> MKIEEVKSTTKTQRIASHSHVKGLGLDESGLAKQAASGLVGQENAREACGVIVELIKSKKMAGRAVLLAGPPGTGKTALALAIAQELGSKVPFCPMVGSEVYSTEIKKTEVLMENFRRAIGLRIKETKEVYEGEVTELTPCETENPMGGYGKTISHVIIGLKTAKGTKQLKLDPSIFESLQKERVEAGDVIYIEANSGAVKRQGRCDTYATEFDLEAEEYVPLPKGDVHKKKEIIQDVTLHDLDVANARPQGGQDILSMMGQLMKPKKTEITDKLRGEINKVVNKYIDQGIAELVPGVLFVDEVHMLDIECFTYLHRALESSI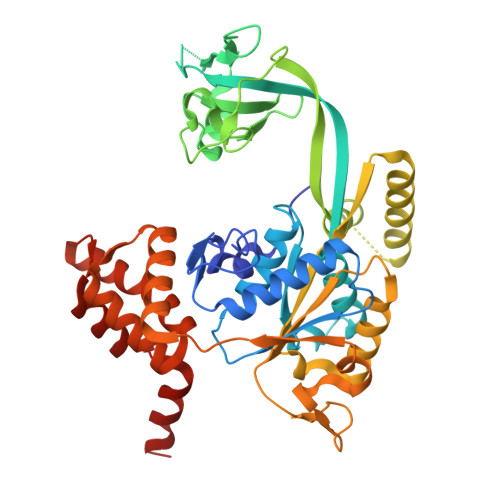APIVIFASNRGNCVIRGTEDITSPHGIPLDLLDRVMIIRTMLYTPQEMKQIIKIRAQTEGINISEEALNHLGEIGTKTTLRYSVQLLTPANLLAKINGKDSIEKEHVEEISELFYDAKSSAKILADQQ>MPMILGYWDIRGLAHAIRLLLEYTDSSYEEKKYTMGDAPDYDRSQWLNEKFKLGLDFPNLPYLIDGAHKITQSNAILCYIARKHNLCGETEEEKIRVDILENQTMDNHMQLGMICYNPEFEKLKPKYLEELPEKLKLYSEFLGKRPWFAGNKITFVDFLVYDVLDLHRIFEPKCLDAFPNLKDFISRFEGLEKISAYMKSS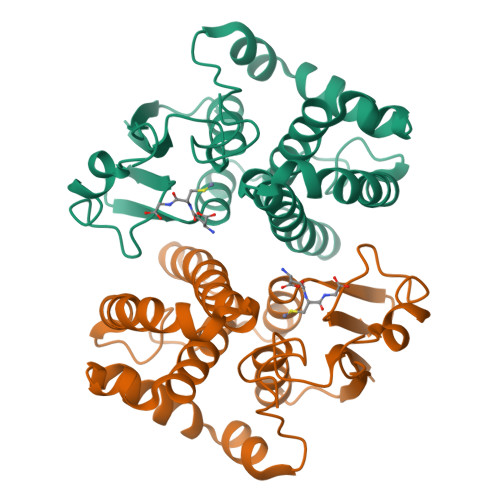RFLPRPVFSKMAVWGNK[3x]9-DEAZAHYPOXANTHINE | C6 H5 N3 O | 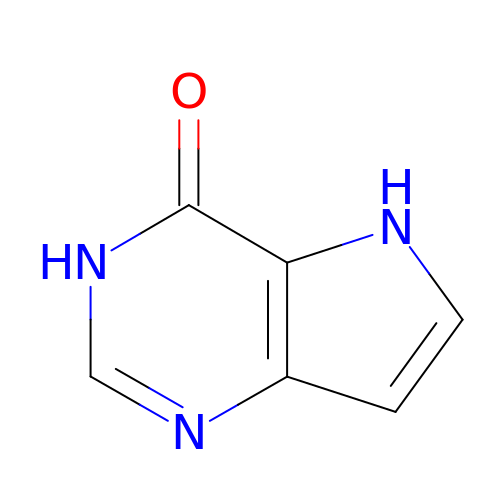UWMXUDUWVFWJPX-UHFFFAOYSA-N6-[(~{Z})-2-(diethylamino)ethenyl]-~{N}-phenyl-7~{H}-purin-2-amine 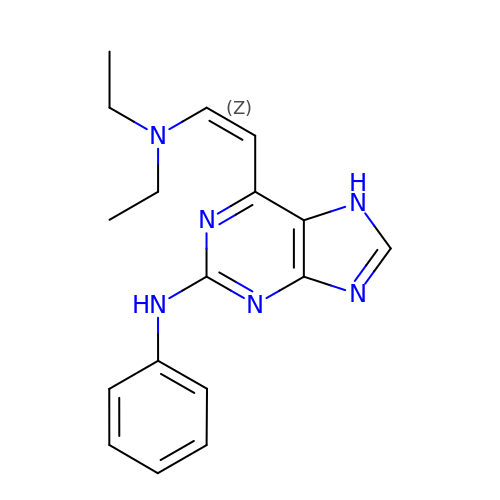| C17 H20 N6 | SHKLUCMYFCYADL-KHPPLWFESA-N> MAQDALSDGFVRLCIDPSLNFFGEGCKILVEGQITDDATAAENVVTCVNSELDLVERFGQGSVLTESLRKVFCMCKSGVSVYALPRADAAAAVSAVYTLTVTGTALTDGRVQLYMGEAEYSLDIGVDEGDTPTQIAAKIVAAISPDFPYEATAAAGVITLTARNG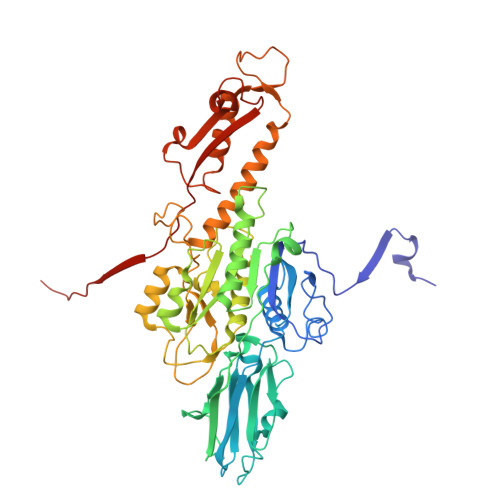GTIGNHLSVIYTNLGSCTSVTPEGVTVAFAQTTPGSVNPEPNDYASVVNECCFAVYVLSSDDTDWQENLRDWIRSAWDCSKPQCFGHGYVFNKGTLGQVLADGDNSAELSRLALPTTYPVLPYLTNAAYGALSACSTCENPELNVQGQTYGLLSCINMPESCTPGWEFTEVTQLQNNGFVVSGPATTSGQGNFTSPYIYNDVTNYLRDEKNRPNATFRDASSRRLAAATGVALATFLQQFNGLAVFTKNTNIKTGIIGTNLRLMLGKIRKWASDNVGVLFSEFDNINEDIQLVSDFDVQPKCVGQPGVFHLNMRYRPPVRGARINVNLVPALFDNCDR3-cyclopropyl-5-[(3R)-pyrrolidin-3-yl]-1,2,4-oxadiazole | C9 H13 N3 O | 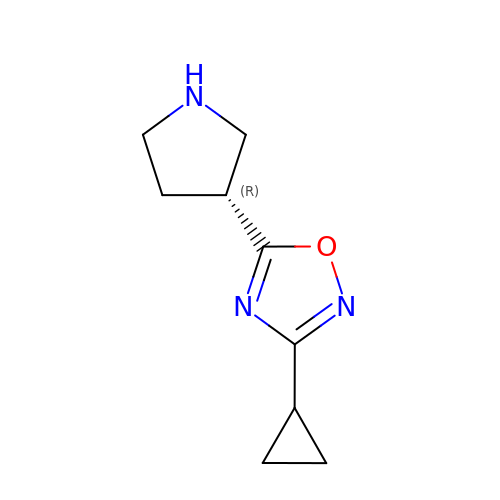UHWKRAJPWOGTQP-SSDOTTSWSA-N> MAGRGSLLRQCPLLLPQNREGTAYEGFVSAQGRDFHIRILLPTDSQLKNARIECSWHLKKILHGYQHILKQRLHSCPDLVSFVVELKTILEIALKNTQELHVPWPPEYYSCLIRDLEILGWNKVAYVDTGLTTVKLKAEDSRGRQHLITLKLNAKYPTEPPDCVVDFPVQFAISWMPQDSLIDIHNQFLAALESLKEFWDTMDEIDGKTWVLEPENPARCATSRRIAIGNNVSVNIEVDPRHPKMLPECYFLGADHAVN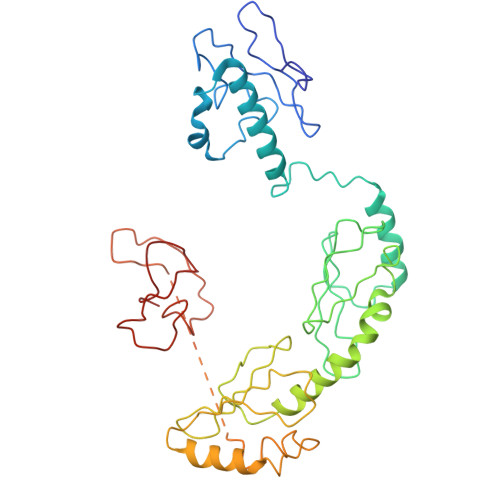PLRTKLNNNMHLWDPEISLLQNLKDLLEIDFPSRAALEKSDFTKDCGICYAYRLNGTTPDQVCNEPRCGQPFHQACLYEWLQGLPSSRQSFNVIFGECPYCNKPLTVKSSMKKP Ferredoxins are small iron–sulfur proteins and key players in essential metabolic pathways. For catalysis, CYPs required electrons typically supplied by redox proteins, such as ferredoxins. Interestingly, two Mtb 3Fe–4S ferredoxins, Fdx and FdxE, are co-located in respective operons with cytochrome P450 (CYP) enzymes suggesting their functional relevance. Here, we explored the genome context for two ferredoxins, Fdx and FdxE, determined the binding kinetics between FdxE and CYP143, and solved three crystal structures: Fdx, CYP143, and a complex FdxE–CYP143.

We constructed a single protein containing FdxE fused via a linker to the N-term of CYP143. This protein was used to obtain a crystal structure of the FdxE−CYP143 complex at 1.6 Å resolution as well as for SAXS studies in solution. In the structure, FdxE binds to the proximal surface of CYP143 and has a typical fold of monocluster ferredoxins for Fdx. The buried area upon the complex formation between FdxE and CYP is 1,809 Å2. The shortest distance between the CYP143 heme group and the ferredoxin iron–sulfur cluster is 16.75 Å. As expected, several structural regions from the CYP143 proximal side participate in a complex formation, namely, helices C, K, and L and the meander preceding the heme-containing loop. The electron density of the iron–sulfur cluster of FdxE clearly identifies a [3Fe–4S] cluster coordinated by Fe—S bonds to cysteines Cys10, Cys16, and Cys54. A residue His13 of the CXXHXXC(X)nCP motif is not ligated to the [3Fe–4S] cluster. Instead, the N1 atom of the imidazole ring of His13 forms a hydrogen bond with the O∑1 atom of Glu56 from the opposite loop around the cluster. The inner salt bridge in the meander, between residues Asp326 and His330, maintains its specific conformation so that Lys328 forms a salt bridge with Asp49 of FdxE.

> MAHHHHHHKVRLDPSRCVGHAQCYAVDPDLFPIDDSGNSILAEHEVRPEDMQLTRDGVAACPEMALILEEDDADVLHRHQPVTIGEPAAKKTTTPGEDHAGSFYLPRLEYSTLPMAVDRGVGWKTLRDAGPVVFMNGWYYLTRREDVLAALRNPKVFSSRKALQPPGNPLPVVPLAFDPPEHTRYRRILQPYFSPAALSKALPSLRRHTVAMIDAIAGRGECEAMADLANLFPFQLFLVLYGLPLEDRDRLIGWKDAVIAMSDRPHPTEADVAAARELLEYLTAMVAERRRNPGPDVLSQVQIGEDPLSEIEVLGLSHLLILAGLDTVTAAVGFSLLELARRPQLRAMLRDNPKQIRVFIEEIVRLEPSAPVAPRVTTEPVTVGGMTLPAGSPVRLCMAAVNRDGSDAMSTDELVMDGKVHRHWGFGGGPHRCLGSHLARLELTLLVGEWLNQIPDFELAPDYAPEIRFPSKSFALKNLPLRWS>MAAAASSA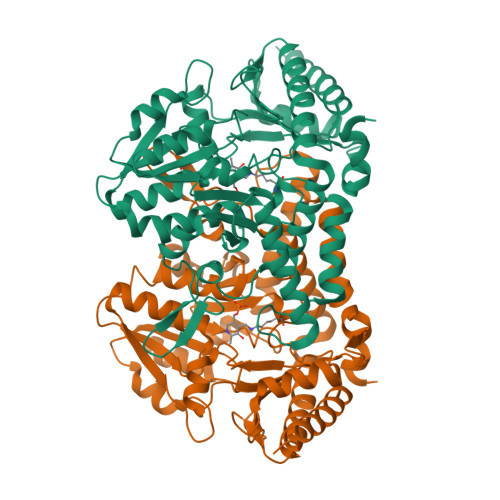TISTDSESVSLGHRVRKDFRILHQEVNGSKLVYLDSAATSQKPAAVLDALQNYYEFYNSNVHRGIHYLSAKATDEFELARKKVARFINASDSREIVFTRNATEAINLVAYSWGLSNLKPGDEVILTVAEHHSCIVPWQIVSQKTGAVLKFVTLNEDEVPDINKLRELISPKTKLVAVHHVSNVLASSLPIEEIVVWAHDVGAKVLVDACQSVPHMVVDVQKLNADFLVASSHKMCGPTGIGFLYGKSDLLHSMPPFLGGGEMISDVFLDHSTYAEPPSRFEAGTPAIGEAIALGAAVDYLSGIGMPKIHEYEVEIGKYLYEKLSSLPDVRIYGPRPSESVHRGALCSFNVEGLHPTDLATFLDQQHGVAIRSGHHSAQPLHRYLGVNASARASLYFYNTKDDVDAFIVALADTVSFFNSFK[2x]> MSNISRQAYADMFGPTVGDKVRLADTELWIEVEDDLTTYGEEVKFGGGKVIRDGMGQGQMLAADCVDLVLTNALIVDHWGIVKADIGVKDGRIFAIGKAGNPDIQPNVTIPIGAATEVIAAEGKIVTAGGIDTHIHWICPQQAEEALVSGVTTMVGGGTGPAAGTHATTCTPGPWYISRMLQAADSLPVNIGLLGKGNVSQPDALREQVAAGVIGLKIQEDWGATPAAIDCALTVADEMDIQVALHSDTLNESGFVEDTLAAIGGRTIHTFHTEGAGGGHAPDIITACAHPNILPSSTNPTLPYTLNTIDEHLDMLMVCHHLDPDIAEDVAFAESRIRRETIAAEDVLHDLGAFSLTSSDSQAMGRVGEVILRTWQVAHRMKVQRGALAEETGDNDNF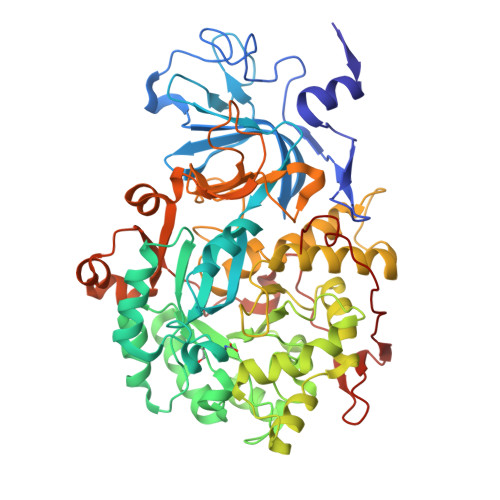RVKRYIAKYTINPALTHGIAHEVGSIEVGKLADLVVWSPAFFGVKPATVIKGGMIAIAPMGDINASIPTPQPVHYRPMFGALGSARHHCRLTFLSQAAAANGVAERLNLRSAIAVVKGCRTVQKADMVHNSLQPNITVDAQTYEVRVDGELITSEPADVLPMAQRYFLF>[900x]MADVTGIALGMIETRGLVPAIEAADAMTKAAEVRLVGRQFVGGGYVTVLVRGETGAVNAAVRAGADACERVGDGLVAAHIIARVHSEVENILPKAPQA;>[60x]MKIMQVEKTLVSTNRIADMGHKPLLVVWEKPGAPRQVAVDAIGCIPGDWVLCVGSSAAREAAGSKSYPSDLTIIGIIDQWNGE;>MPSQSGMNPADLSGLSGKELARARRAALSKQGKAAVSNKTASVNRSTKQAASSINTNQVRSSVNEVPTDYQMADQLCSTIDHADFGTESNRVRDLCRQRREALSTIGKKAAKTTGKPSGRVRPQQSVVHNDAMIENAGDTNQSSSTSLNNELSEICSIADDMPERFGSQAKTVRDICRARRQALSERGTRAVPPKPQSQGGPGRNGYQIDGYLDTALHGRDAAKRHREMLCQYGRGTAPSCKPTGRVKNSVQSGNAAPKKVETGHTLSGGSVTGTQVDRKSHVTGNEPGTCRAVTGTEYVGTEQFTSFCNTSPKPNATKVNVTTTARGRPVSGTEVSRTEKVTGNESGVCRNVTGTEYMSNEAHFSLCGTAAKPSQADKVMFGATARTHQVVSGSDEFRPSSVTGNESGAKRTITGSQYADEGLARLTINGAPAKVARTHTFAGSDVTGTEIGRSTRVTGDESGSCRSISGTEYLSNEQFQSFCDTKPQRSPFKVGQDRTNKGQSVTGNLVDRSELVTGNEPGSCSRVTGSQYGQSKICGGGVGKVRSMRTLRGTSVSGQQLDHAPKMSGDERGGCMPVTGNEYYGREHFEPFCTSTPEPEAQSTEQSLTCEGQIISGTSVDASDLVTGNEIGEQQLISGDAYVGAQQTGCLPTSPRFNQTGNVQSMGFKNTNQPEQNFAPGEVMPTDFSIQTPARSAQNRITGNDIAPSGRITGPGMLATGLITGTPEFRHAARELVGSPQPMAMAMANRNKAAQAPVVQPEVVATQEKPELVCAPRSDQMDRVSGEGKERCHITGDDWSVNKHITGTAGQWASGRNPSMRGNARVVETSAFANRNVPKPEKPGSKITGSSGNDTQGSLITYSGGARG[120x]

Carboxysomes are specialized microcompartments found in all cyanobacteria and certain chemoautotrophic proteobacteria, playing a crucial role in CO2 fixation and serving as a central component of bacterial CO2-concentrating mechanisms. These organelles encapsulate 2 cargo enzymes: Ribulose-1,5-bisphosphate carboxylase/oxygenase (Rubisco) and carbonic anhydrase, using a polyhedral proteinaceous shell. Self-assembly of the α-carboxysome is mediated by the intrinsically disordered protein CsoS2. CsoS2 functions as a linker protein, connecting cargo enzymes like Rubisco with the shell proteins.

To address this issue, we reanalyzed our recently reported cryo-EM density maps without applying any symmetry (C1 symmetry). Fortunately, we were still able to obtain maps for the T = 9 and T = 16 α-carboxysome shells at resolutions of 2.77 Å and 3.71 Å, respectively. The construction of structures using C1 symmetry maps yielded T = 9 shells with a diameter of 36.9 nm and T = 16 shells with a diameter of 49.2 nm, which are virtually identical to the structures obtained under I symmetry. Intriguingly, we observed a complete and continuous density at the centroid of the inner surface along the 3-fold axis within the T = 16 shell C1 symmetry map, whereas the corresponding position in the I symmetry map showed only limited weaker, fragmented densities. Specifically, this relative position coincides with the junction of 3 copies and the 3-fold axis under I symmetry, suggesting that the density discrepancies at the same position in maps of different symmetries are due to symmetrical treatment. High-symmetry processing involves a high degree of data averaging, which can lead to the fragmentation or even the absence of complete density. Based on the relative position and conformation of this density on the inner surface of the α-carboxysome shell, we have reason to identify it as the density of CsoS2. Although we were only able to partially build the structure of CsoS2 from Ser710 to Thr721 owing to distortions in the density caused by superposition and averaging of the particles during cryo-EM data processing, this result is a meaningful complement to unveiling the distribution of CsoS2 on the inner surface of the α-carboxysome shell. The results of this study indicate that there are also potential CsoS2-binding sites at the threefold axis of the facet of larger shells (with a diameter >44.5 nm), thereby augmenting the theoretical number of CsoS2 molecules within a single shell. Furthermore, the comparison of maps under C1 and I symmetry reveals additional CsoS2-binding sites on the inner surface of the α-carboxysome shell.>[6x]MKLIILEHYSQASEWAAKYIRNRIIQFNPGPEKYFTLGLPTGSTPLGCYKKLIEYYKNGDLSFKYVKTFNMDEYVGLPRDHPESYHSFMWNNFFKHIDIHPENTHILDGNAVDLQAECDAFEEKIKAAGGIELFVGGIGPDGHIAFNEPGSSLVSRTRVKTLAMDTILANARFFDGELTKVPTMAL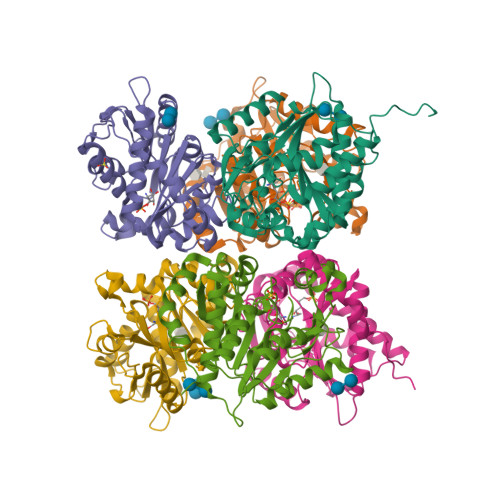TVGVGTVMDAREVMILITGAHKAFALYKAIEEGVNHMWTVSAFQQHPRTVFVCDEDATLELKVKTVKYFKGLMLVHNKLVDPLYSIKEKETEKSQSSKKPYSD>CACCGAGCG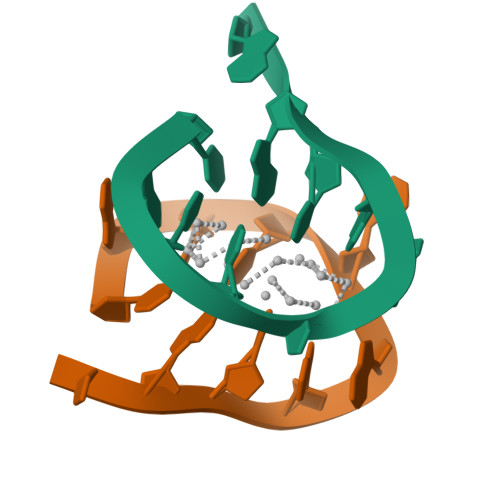A[2x]> XITID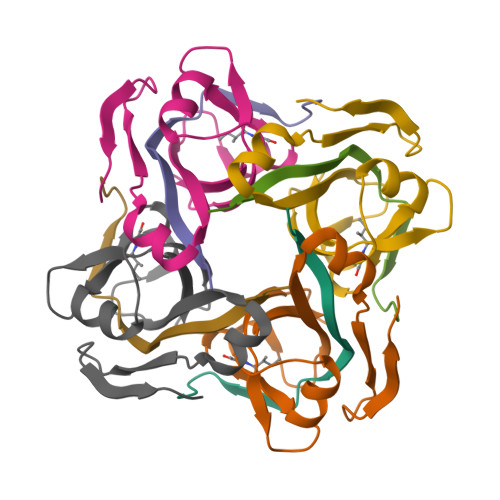EDLAKLAKLREGMKVEIVDVNNGERFSTYVILGKKRGEICVNGAAARKVAIGDVVIILAYASMNEDEINAHKPSIVLVDEKNEILEKGLEH;> MTFEMLYSKIHRATITDANLNYIG6-({4-[(3S)-3-cyano-3-cyclopropyl-2-oxopyrrolidin-1-yl]pyridin-2-yl}amino)-N,N-dimethylpyridine-3-carboxamide 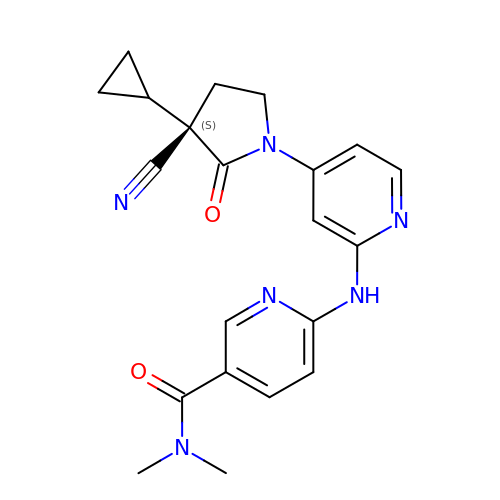| C21 H22 N6 O2 | CFHPNFDEUWSEIR-OAQYLSRUSA-N>[6x]MHHHHHHMNSEALGMIETKGLVGSIEAADAMVDAANVTLIGKEHVGGGLVTV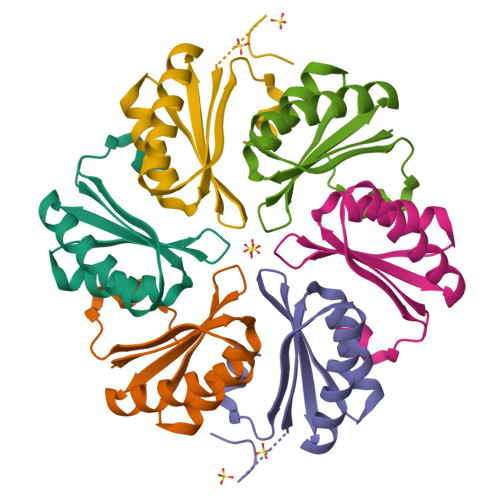LVRGDVGAVKAATDAGAAAAQRVGELVSVHVIPRPHIEVETILPHSK>[60x]MKAFEFLYEDFQRGLTVVLDKGLPPKFVEDYLKVCGDYIDFVKFGWGTSAVIDRDVVKEKINYYKDWGIKVYPGGTLFEYAYSKGEAAEFIAECKKLGFEAVEISDGSSDISLDDRKAAIWGAKWAGFMVLTEVGKKMPDKDKQLTIDDRIKLINFDLDAGADYVIIEGRESGKGIGLFDKEGKVKENELDVLAKNVDINKVIFEAPQKSQQVAFILKFGSSVNLANIAFDEVISLETLRRGLRGDTFGKVLEHHHHHH

Here, we develop a general method for designing self-assembling proteins that uses predicted structures of oligomeric proteins from thermophilic organisms as building blocks. Of the 359 identified thermophilic trimer homologs, 191 yielded high-confidence AF2 predictions [predicted aligned error (pAE) < 5, predicted local distance difference test (pLDDT) > 90]. We docked these predicted structures in the so-called “I3” architecture by aligning their threefold symmetry axes to the corresponding axes of icosahedral point group symmetry, using the Rosetta SymDofMover to sample the translational and rotational degrees of freedom along this shared axis [Fig. 1C, (27)]. To evaluate the accuracy of our design method at high resolution, we used single-particle cryoelectron microscopy (cryo-EM) to determine the structures of one nanoparticle from each of the successful PDB seeds.

We measured the aggregation temperature (Tagg) for each nanoparticle by monitoring DLS while heating from 25 to 84 °C, which showed that all nanoparticles retained their intended assembly state until at least 60 °C, and I3-D12 did not aggregate in the measured range. Icosahedral 3D reconstructions at 2.5 Å, 2.3 Å, and 3.5 Å resolution were obtained for I3-A6, I3-D12, and I3-A7, respectively, allowing us to build atomic models of each nanoparticle. Comparing the experimental cryo-EM structures to the computational design models demonstrated that AF2 structure prediction was quite accurate: The all-atom rmsd for a single monomer of I3-A6, I3-D12, and I3-A7 were 1.3 Å, 1.7 Å, and 1.4 Å, respectively. Aligning two subunits across the designed interfaces revealed that these were designed with high accuracy, yielding alpha-carbon rmsds of 0.7 Å, 1.1 Å, and 1.5 Å, respectively. In each case, the rotameric states of the interdigitated hydrophobic side chains at the designed interfaces corresponded well with the design models, as did the polar residues lining the periphery of the I3-A6 and I3-D12 interfaces. Slight rigid body deviations between the building blocks added up to alpha-carbon rmsds of 1.6 Å, 2.2 Å, and 2.2 Å across the entire 60-subunit nanoparticle for I3-A6, I3-D12, and I3-A7, respectively. These values are comparable to those obtained from previous computational nanoparticle design campaigns that started from high-resolution crystal structures of the building blocks.>[2x]MRSSLAPGVWFFRAFSRDSWFRGLILLLTFLIYACYHMSRKPISIVKSRLHQNCSEQIKPINDTHSLNDTMWCSWAPFDKDNYKELLGGVDNAFLIAYAIGMFISGVFGERLPLRYYLSAGMLLSGLFTSLFGLGYFWNIHELWYFVVIQVCNGLVQTTGWPSVVTCVGNWFGKGKRGFIMGIWNSHTSVGNILGSLIAGIWVNGQWGLSFIVPGIITAVMGVITFLFLIEHPEDVDCAPPQHHGEPAE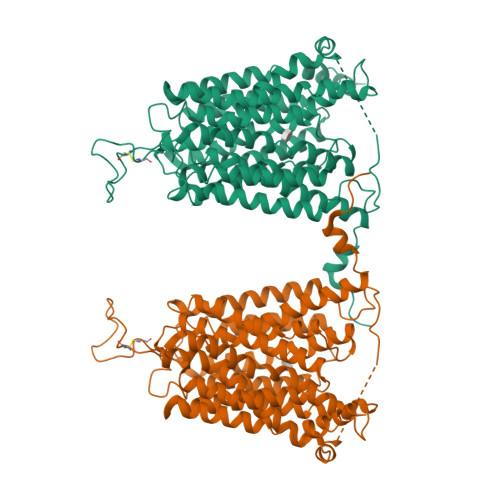NQDNPEDPGNSPCSIRESGLETVAKCSKGPCEEPAAISFFGALRIPGVVEFSLCLLFAKLVSYTFLYWLPLYIANVAHFSAKEAGDLSTLFDVGGIIGGIVAGLVSDYTNGRATTCCVMLILAAPMMFLYNYIGQDGIASSIVMLIICGGLVNGPYALITTAVSADLGTHKSLKGNAKALSTVTAIIDGTGSIGAALGPLLAGLISPTGWNNVFYMLISADVLACLLLCRLVYKEILAWKVSLSRGSGYKEI>[2x]ILEAAVTQSPRNKVAVTGEKVTLSCQQTNNHNNMYWYRQDT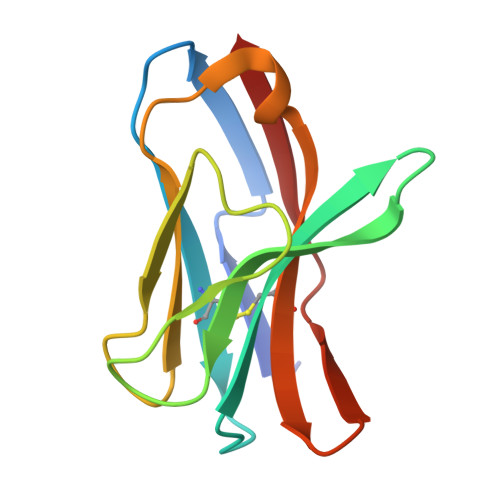GHGLRLIHYSYGAGNTEKGDIPDGYEASRPSHEQFSLILVSATPSQSSVYFCASGVGGTLYFGAGTRLSVL(5S)-5-[(6R)-6-hydroxy-6-methyl-5-oxooctyl]furan-2(5H)-one | C13 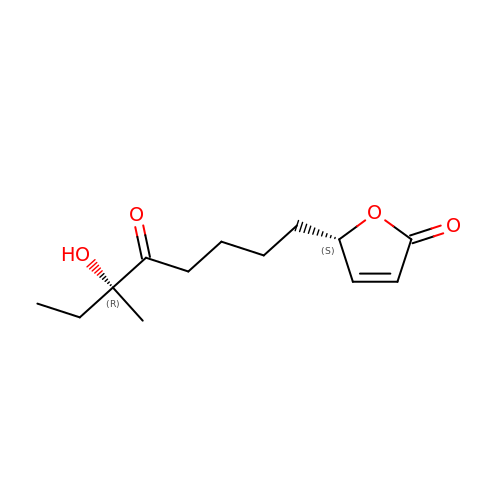H20 O4 | UOBYXVHBYDUQMN-GXFFZTMASA-N> IVGGQECKDGECPWQALLINEENEGFCGGTILSEFYILTAAHCLYQAKRFKVRVGDRNTAAEEGGEAVHEVEVVIKHNRFTKETYDFDIAVLRLKTPITFRMNVAPACLPERDWAESTLMTQKTGIVSGFGRTHEK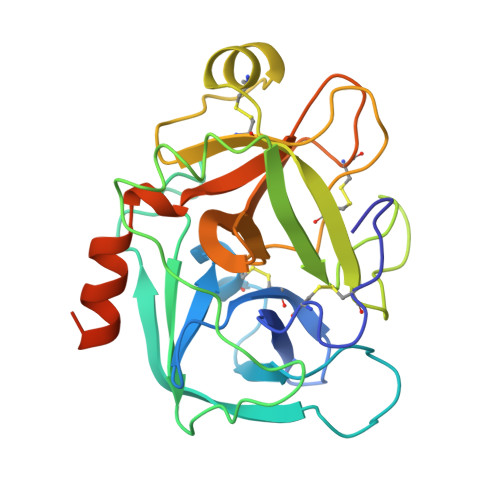GRQSTRLKMLEVPYVDRNSCKLSSSFIITQNMFCAGYDTKQEDACQGDSGGPHVTRFKDTYFVTGIVSWGEGCARKGKYGIYTKVTAFLKWIDRSMKTRGLPKAKSHAPEVITSSPLK> MRT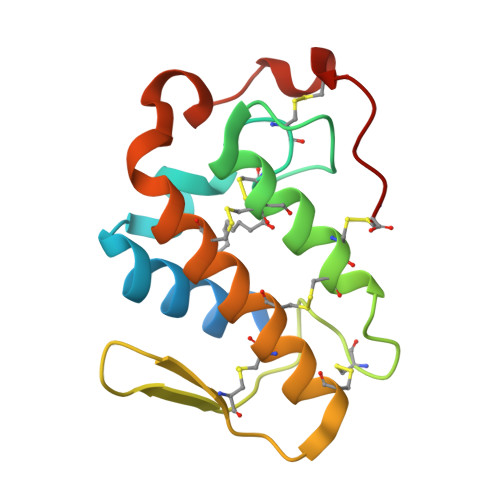LWIMAVLLVGVEGSLVELGKMILQETGKNPVTSYGAYGCNCGVLGRGKPKDATDRCCSVHKCCYKKMTGCNPKKDRYSYSWKDKTIVCDENNPCLKELCECDKAVAICLRENLDTYNEKYKKYYKKPLCKKADPC> MSRESNDTIQSDTVRSSSKSDYFRIQLNNQDYYMSKPTFLDPSHGESLPLNQFSQVPNIRVFGALPTGHQVLCHVHGILPYMFIKYDGQITDTSTLRHQRCAQVHKTLEVKIRASFKRKKDDKHDLAGDKLGNLNFVADVSVVKGIPFYGYHVGWNLFYKISLLNPSCLSRISELIRDGKIFGKKFEIYESHIPYLLQWTADFNLFGCSWINVDRCYFRSPVLNSILDIDKLTINDDLQLLLDRFCDFKCNVLSRRDFPRVGNGLIEIDILPQFIKNREKLQHRDIHHDFLEKLGDISDIPVKPYVSSARDMINELTMQREELSLKEYKEPPETKRHVSGHQWQSSGEFEAFYKKAQHKTSTFDGQIPNFENFIDKNQKFSAINTPYEALPQLWPRLPQIEINNNSMQDKKNDDQVNASFTEYEICGVDNENEGVKGSNIKSRSYSWLPESIASPKDSTILLDHQTKYHNTINFSMDCAMTQNMASKRKLRSSVSANKTSLLSRKRKKVMAAGLRYGKRAFVYGEPPFGYQDILNKLEDEGFPKIDYKDPFFSNPVDLENKPYAYAGKRFEISSTHVSTRIPVQFGGETVSVYNKPTFDMFSSWKYALKPPTYDAVQKWYNKVPSMGNKKTESQISMHTPHSKFLYKFASDVSGKQKRKKSSVHDSLTHLTLEIHANTRSDKIPDPAIDEVSMIIWCLEEETFPLDLDIAYEGIMIVHKASEDSTFPTKIQHCINEIPVMFYESEFEMFEALTDLVLLLDPDILSGFEIHNFSWGYIIERCQKIHQFDIVRELARVKCQIKTKLSDTWGYAHSSGIMITGRHMINIWRALRSDVNLTQYTIESAAFNILHKRLPHFSFESLTNMWNAKKSTTELKTVLNYWLSRAQINIQLLRKQDYIARNIEQARLIGIDFHSVYYRGSQFKVESFLIRICKSESFILLSPGKKDVRKQKALECVPLVMEPESAFYKSPLIVLDFQSLYPSIMIGYNYCYSTMIGRVREINLTENNLGVSKFSLPRNILALLKNDVTIAPNGVVYAKTSVRKSTLSKMLTDILDVRVMIKKTMNEIGDDNTTLKRLLNNKQLALKLLANVTYGYTSASFSGRMPCSDLADSIVQTGRETLEKAIDIIEKDETWNAKVVYGDTDSLFVYLPGKTAIEAFSIGHAMAERVTQNNPKPIFLKFEKVYHPSILISKKRYVGFSYESPSQTLPIFDAKGIETVRRDGIPAQQKIIEKCIRLLFQTKDLSKIKKYLQNEFFKIQIGKVSAQDFCFAKEVKLGAYKSEKTAPAGAVVVKRRINEDHRAEPQYKERIPYLVVKGKQGQLLRERCVSPEEFLEGENLELDSEYYINKILIPPLDRLFNLIGINVGNWAQEIVKSKRASTTTTKVENITRVGTSATCCNCGEELTKICSLQLCDDCLEKRSTTTLSFLIKKLKRQKEYQTLKTVCRTCSYRYTSDAGIENDHIASKCNSYDCPVFYSRVKAERYLRDNQSVQREEALISLNDW;>MNRWVEKWLRVYLKCYINLILFYRNVYPPQSFDYTTYQSFNLPQFVPINRHPALIDYIEELILDVLSKLTHVYRFSICIINKKNDLCIEKYVLDFSELQHVDKDDQIITETEVFDEFRSSLNSLIMHLEKLPKVNDDTITFEAVINAIELELGHKLDRNRRVDSLEEKAEIERDSNWVKCQEDENLPDNNGFQPPKIKLTSLVGSDVGPLIIHQFSEKLISGDDKILNGVYSQYEEGESIFGSLF[2x];> LHMDALLTKFNEDRSLQDENLSQPRTRVRIVDDNLYNKSNPFQLCYKKRDYGSQYYHIYQYRLKTFRERVLKECDKRWDAGFTLNGQLVLKKDKVLDIQGNQPCWCVGSIYCEMKYKPNVLDEVINDTYGAPDLTKSYTDKEGGSDEIMLEDESGRVLLVGDFIRSTPFITGVVVGILGMEAEAGTFQVLDICYPTPLPQNPFPAPIATCPTRGKIALVSGLNLNNTSPDRLLRLEILREFLMGRINNKIDDISLIGRLLICGNSVDFDIKSVNKDELMISLTEFSKFLHNILPSISVDIMPGTNDPSDKSLPQQPFHKSLFDKSLESYFNGSNKEILNLVTNPYEFSYNGVDVLAVSGKNINDICKYVIPSNDNGESENKVEEGESNDFKDDIEHRLDLMECTMKWQNIAPTAPDTLWCYPYTDKDPFVLDKWPHVYIVANQPYFGTRVVEIGGKNIKIISVPEFSSTGMIILLDLETLEAETVKIDI;> MDQKASYFINEKLFTEVKPVLFTDLIHHLKIGPSMAKKLMFDYYKQTTNAKYNCVVICCYKDQTIKIIHDLSNIPQQDSIIDCFIYAFNPMDSFIPYYDIIDQKDCLTIKNSYELKVSESSKIIERTKTLEEKSKPLVRPTARSKTTPEETTGRKSKSKDMGLRSTALLAKMKKDRDDKETSRQNELRKRKEENLQKINKQNPEREAQMKELNNLFVEDDLDTEEVNGGSKPNSPKETDSNDKDKNNDDLEDLLETTAEDSLMDVPKIQQTKPSETEHSKEPKSEEEPSSFIDEDGYIVTKRPATSTPPRKPSPVVKRALSSSKKQETPSSNKRLKKQGTLESFFKRKAK

The translesion synthesis (TLS) DNA polymerases Rev1 and Polζ function together in DNA lesion bypass during DNA replication, acting as nucleotide inserter and extender polymerases, respectively. It belongs to the B family of polymerases and is composed of subunits Rev3, Rev7, Pol31, and Pol32 (24, 25). The Polζ subunit Rev7 is a hub protein that directly binds Rev1 and is a component of several other protein complexes such as the shieldin DNA double-strand break repair complex. Rev7 is a member of the HORMA (Hop1, Rev7, and Mad2 proteins) domain protein family.

We then used single-particle cryo-EM to visualize the structure of the pentameric apo Polζ holoenzyme comprising two Rev7 subunits and one subunit each of Rev3, Pol31, and Pol32 arranged around a central canal. We obtained a consensus 3D cryo-EM reconstruction at 4.11 Å resolution, determined by the golden standard Fourier-shell correlation (FSC) method at a cutoff of 0.143 (29). The five subunits of apo Polζ organize into a ring-like structure. We can also identify the cryo-EM density of the [4Fe-4S] cluster in Rev3, which is essential to the catalytic activity of Rev3 (31). Upon DNA binding, concerted movements of three Rev3 loops (948–960 aa, 1050–1094 aa, and 1095–1107 aa) increase the size of the DNA-binding channel opening, from a closed to an open state. The channel opening sizes of apo Polζ and Polζ states A and B are 18.2 Å, 20.6 Å, and 20.7 Å, respectively. Our apo structure shows that one lysine residue (K1214) of Rev3 protrudes up and points toward the pore where nucleotide insertion occurs. When a DNA oligomer is present, K1214 moves away from the pore and leaves space for DNA binding. Within the Polζ complex, the two subunits of Rev7, Rev7A, and Rev7B bind the Rev7-binding motifs 1 (RBM1; 517–540 aa) and 2 (RBM2; 599–623 aa) of Rev3, respectively. Our apo Polζ structure shows that the safety belts of Rev7A and Rev7B adopt a closed conformation in their Rev3RBM1-and Rev3RBM2-bound states, respectively.>SLLKLAIPKGRLEEKVMTYLKKTGVIFERESSILREGKDIVCFMVRPFDVPTYLVHGVADIGFCGTDVLLEKETSLIQPFFIPTNISRMVLAGPKGRGIPEGEKRIATKFPNVTQRYCESKGWHCRIIPLKGSVELAPIAGLSDLIVDITETGRTLKENNLEILDEIFVIRTHVVVNPVSYRTKREEVVSFLEKLQEVIEHDSNEQSRGEGGSHHHHHH[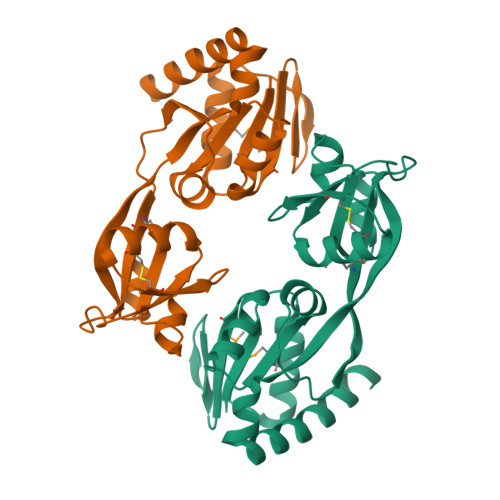2x]>GAMDLLELSDVDSESSDISQPYVVCRQCPEYRRQAAQPPHCPAPEGEPGAPQALGDAPSTSVSLTTAVQDYVCPLQGSHALCTCCFQPMPDRRVEREQDPRVAPQQCAVCLQPFCHLYWGCTRTGC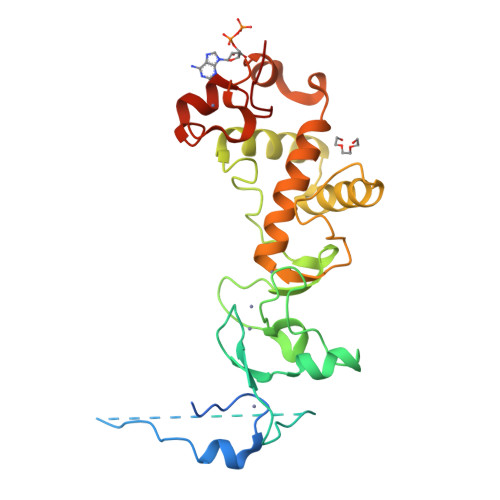YGCLAPFCELNLGDKCLDGVLNNNSYESDILKNYLATRGLTWKNMLTESLVALQRGVFLLSDYRVTGDTVLCYCCGLRSFRELTYQYRQNIPASELPVAVTSRPDCYWGRNCRTQVKAHHAMKFNHICEQTRFKN[2x]Collagen prolyl 4‐hydroxylase (C‐P4H) catalyzes the 4‐hydroxylation of Y‐prolines of the XYG‐repeat of procollagen. The α‐subunit provides the N‐terminal dimerization domain, the middle peptide‐substrate–binding (PSB) domain, and the C‐terminal catalytic (CAT) domain. There are three isoforms of the α‐subunit, complexed with a β‐subunit that is protein disulfide isomerase, forming C‐P4H I‐III. The PSB domain of the α‐subunit binds proline‐rich peptides, but its function with respect to the prolyl hydroxylation mechanism is unknown.

In addition, it is shown here by crystallographic binding studies that the POG‐PAG‐POG peptide (with 4‐hydroxyprolines at Y‐positions 2 and 8) also adopts the PxGP mode of binding to PSB‐I as well as to PSB‐II. Calorimetric binding studies show that the affinities of these peptides are lower for PSB‐I than for PSB‐II, with, respectively, K D values of about 70 μM for PSB‐I and 20 μM for PSB‐II.

>[4x]MSFLTAEDCFELGKVAYTEADYYHTELWMEQALRQLDEGEISTIDKVSVLDYLSYAVYQQGDLDKALLLTKKLLELDPEHQRANGNLKYFEYIMAKELEHHHHHH;>[3x]PPGPAGPPG> GPLGSNNVNDLITVTKQMITEGIKDDGVIQAHDGEHIIYTSDFKIDNAVKAGDTMTVKYDKHTIPSDITDDFTPVDITDPSGEVIAKGTFDLNTKTITYKFTDYVDRYENVNAKLELNSYIDKKEVPNETNLNLTFATADKETSKNVKVEYQKPIVKDESNIQSIFSHLDTTKHEVEQTIYVNPLKLNAKNTNVTIKSGGVADNGDYYTGDGSTIIDSNTEIKVYKVASGQQLPQSNKIYDYSQYEDVTNSVTINKNYGTNMANINFGDIDSAYIVK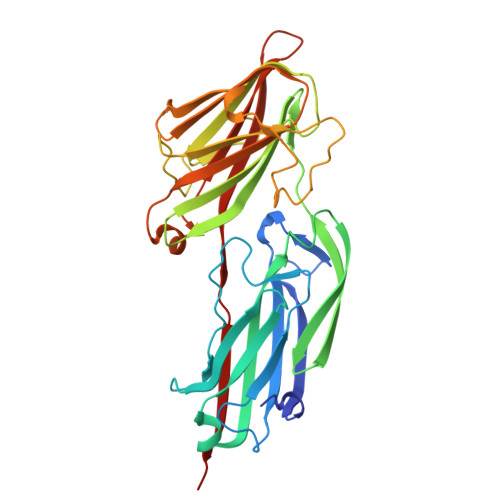VVSKYTPGAEDDLAVQQGVRMTTTNKYNYSSYAGYTNTILSTTDSGGGDGTVKP N-[(BENZYLOXY)CARBONYL]-L-ALANYL-L-PROLINE | C16 H20 N2 O5 | 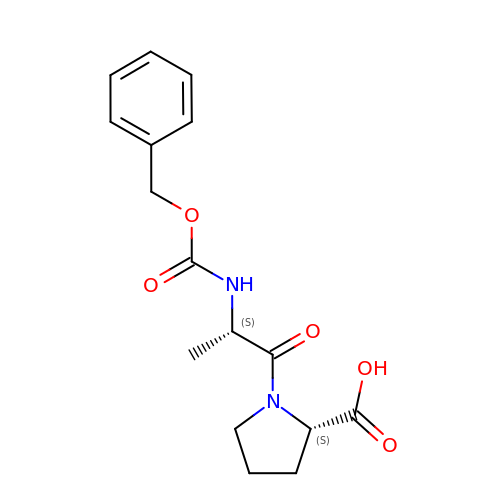RSSOZTMMMIWOJB-AAEUAGOBSA-N> RPPNIVLIFADDLGYGDLGCYGHPSSTTPNLDQLA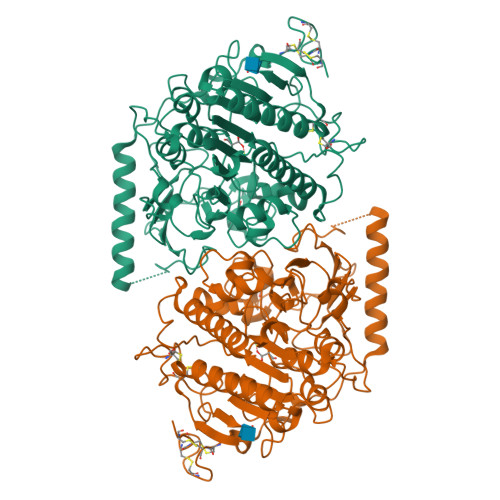AGGLRFTDFYVPVSLATPSRAALLTGRLPVRMGMYPGVLVPSSRGGLPLEEVTVAEVLAARGYLTGMAGKWHLGVGPEGAFLPPHQGFHRFLGIPYSHDQGPCQNLTCFPPATPCDGGCDQGLVPIPLLANLSVEAQPPWLPGLEARYMAFAHDLMADAQREDRPFFLYYASHHTHYPQFSGQSFAERSGRGPFGDSLMELDAAVGTLMTAIGDLGLLEETLVIFTADNGPETMRMSRGGCSGLLRCGKGTTYEGGVREPALAFWPGHIAPGVTHELASSLDLLPTLAALAGAPLPNVTLDGFDLSPLLLGTGKSPRQSLFFYPSYPDEVRGVFAVRTGKYKAHFFTQGSAHSDTTADPACHASSSLTAHEPLLLYDLSKDPGENYNLLGGVAGATPEVLQALKQLQLLKAQLDAAVTFGPSQVARGEDPALQICCHPGCTPRPACCHCPDPHA> MHHHHHHGENLYFQGSSRGMSGLEDSSDLVVSPYVRMGGLTTDPVPTGGDDPHKVAMLGLTFDDVLLLPAASDVVPATADTSSQLTKKIRLKVPLVSSAMDTVTESRMAIAMARAGGMGVLHRNLPVAEQAGQVEMVKRSGGLLVGAAVGVGGDAWVRAMMLVDAGVD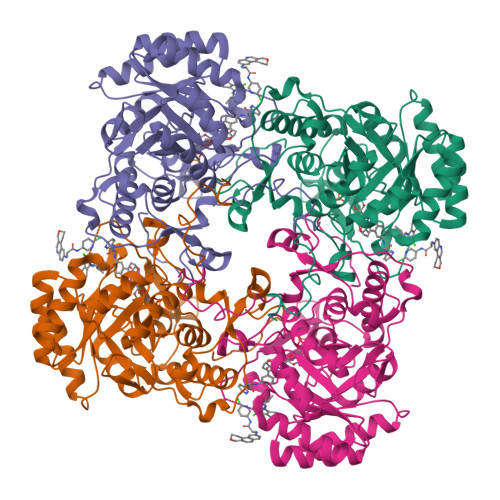VLVVDTAHAHNRLVLDMVGKLKSEVGDRVEVVGGNVATRSAAAALVDAGADAVKVGVGPGSICTTRVVAGVGAPQITAILEAVAACRPAGVPVIADGGLQYSGDIAKALAAGASTAMLGSLLAGTAEAPGELIFVNGKQYKSYRGMGSLGAMRGRGGATSYSKDRYFADDALSEDKLVPEGIEGRVPFRGPLSSVIHQLTGGLRAAMGYTGSPTIEVLQQAQFVRITPAGLKESHPHDVAMTVEAPNYYARGNS> HGMSQPACTARRRTRVLILGVNGFIGNH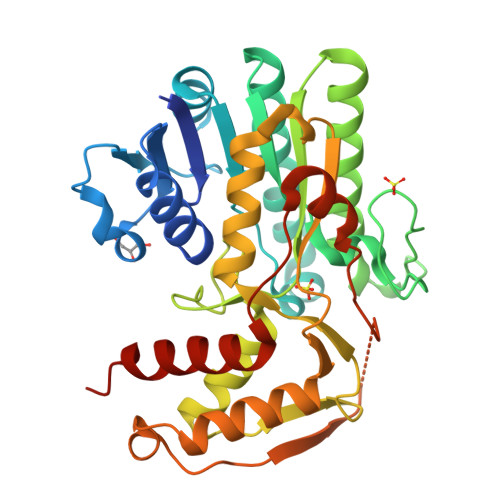LTERLLREDHYEVYGLDIGSDAISRFLNHPHFHFVEGDISIHSEWIEYHVKKCDVVLPLVAIATPIEYTRNPLRVFELDFEENLRIIRYCVKYRKRIIFPSTAEVYGMCSDKYFDEDHSNLIVGPVNKPRWIYSVSKQLLDRVIWAYGEKEGLQFTLFRPFNWMGPRLDNLNAARIGSSRAITQLILNLVEGSPIKLIDGGKQKRCFTDIRDGIEALYRIIENAGNRCDGEIINIGNPENEASIEELGEMLLASFEKHPLRHHFPPFAGFRVVESSSYYGKGYQDVEHRKPSIRNAHRCLDWEPKIDMQETIDETLDFFLRTVDLTDKPS> GSHMKNSVSVDLPGSMKVLVSKSSNADGKYDLIATVDALELSGTSDKNNGSGVLEGVKADASKVKLTISDDLGQTTLEVFKSDGSTLVSKKVTSG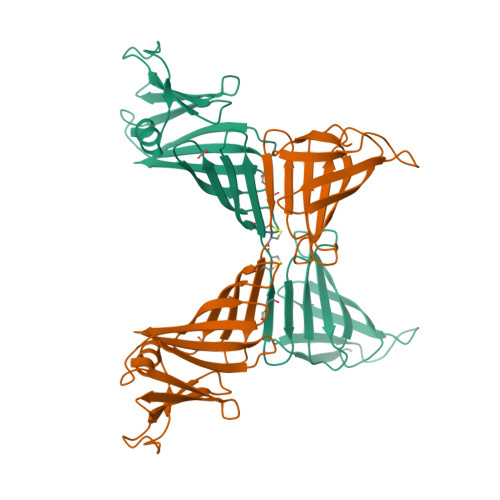GSSTEEKCTCEKIITRADGTRLEYTGIKSDGSGKAKEVLKGYVLEGTLTAEKTTLVVKEGTVTLSKNISKSGEVSVELNDTDSSAATKKTAAWNSGTSTLTITVNSKKTKDLVFTSSNTITVQQYDSNGTSLEGSAVEITKLDEIKNALK> RQEETKKDYREVEKLLRAVADGDLEMVRYLLEWTEEDLEDAEDTVSAADPEFCHPLCQCPKCAPAQKRLAKVPASGLGVNVTSQDGSSPLHVAALHGRADLIPLLLKHGANAGARNADQAVPLHLACQQGHFQVVKCLLDSNAKPNKKDLSGNTPL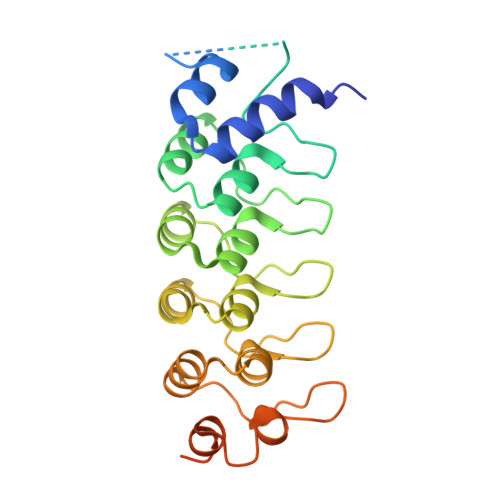IYACSGGHHELVALLLQHGASINASNNKGNTALHEAVIEKHVFVVELLLLHGASVQVLNKRQRTAVDCAEQNSKIMELLQVVPSCVASLDDVAETDRKEYVTVKIRKHHHHHH> MKKEKIDLFYGALLHNIGKVIQRATGERKKHALVGADWFDEIADNQVISDQIRYHMANYQSDKLGNDHLAYITYIADNIASGVDRRQSNEESDEDTSAKIWDTYTNQADIFNVFGAQTDKRYFKPTVLNLKSKPNFASATYEPFSKGDYAAIATRIKNELAEFEFNQVQIDSLLNLFEATLSFVPSSTNTKEIADISLADHSRLTAAFALAIYDYLEDKGRHNYKEDLFTKVSAFYEEEAFLLASFDLSGIQDFIYNINIATNGAAKQLKARSLYLDFMSEYIADSLLDKLGLNRANMLYVGGGHAYFVLANTEKTVETLVQFEKDFNQFLLANFQTRLYVAFGWGSFAAKDIMSELNSPESYRQVYQKASRMISKKKISRYDYQTLMLLNRGGKSSERECEICHSVENLVSYHDQKV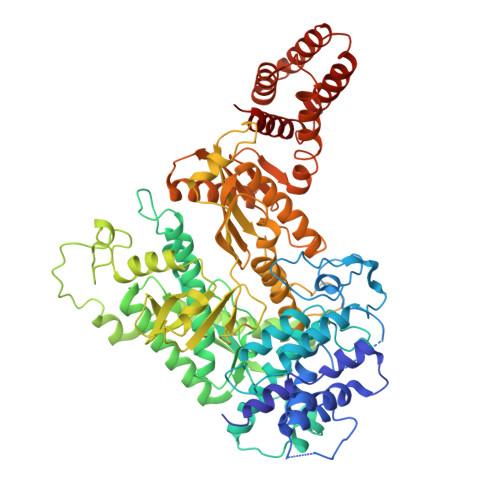CDICRGLYQFSKEIAHDHFIITENEGLPIGPNACLKGVAFEKLSQEAFSRVYVKNDYKAGTVKATHVFVGDYQCDEIYNYAALSKNENGLGIKRLAVVRLDVDDLGAAFMAGFSQQGNGQYSTLSRSATFSRSMSLFFKVYINQFASDKKLSIIYAGGDDVFAIGSWQDIIAFTVELRENFIKWTNGKLTLSAGIGLFADKTPISLMAHQTGELEEAAKGNEKDSISLFSSDYTFKFDRFITNVYDDKLEQIRYFFNHQDERGKNFIYKLIELLRNHDRMNMARLAYYLTRLEELTRETDRDKFKTFKNLFYSWYTNKNDKDRKEAELALLLYIYEIRKD>[2x]VPPPLTPVADVVRPSAAEEARTIAASTNVGTLATLTTEGDPWASFVTYGLLGGAPVLCVSDMAEHGRNLAHDPRASIAIVAPSAESDPLASARVTLAGVAERPEGDELAAARAAHLDAVAAA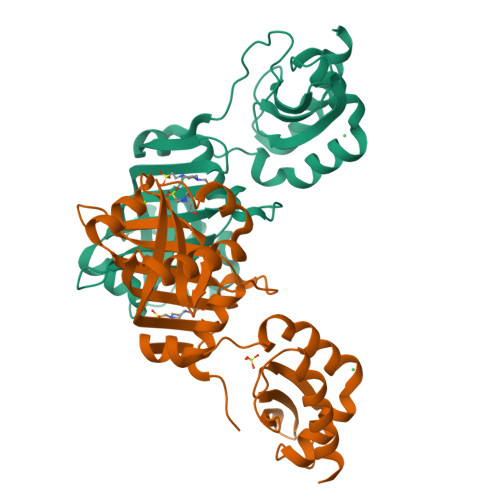KYYIDYSDFSVWVLRVQRVRWVGGYGRMDSTTGEAYAAAEADPVTPRAAGAIAHLNADHADSLLAMARNLGGYPDTGEAVCTGADRYGLDLRVTTERGVAYTRVGYAAPISSFDQLRAATVELAQRAKQS>[2x]MSDAAPSLSNLFYDPTYNPGQSTINYTSIYGNGSTITFDELQGLVNSTVTQAIMFGVRCGAAALTLIVMWMTSRSRKTPIFIINQVSLFLIILHSALYFKYLLSNYSSVTYALTGFPQFISRGDVHVYGATNIIQVLLVASIETSLVFQIKVIFTGDNFKRIGLMLTSISFTLGIATVTMYFVSAVKGMIVTYNDVSATQDKYFNASTILLASSINFMSFVLVVKLILAIRSRRFLGLKQFDSFHILLIMSCQSLLVPSIIFILAYSLKPNQGTDVLTTVATLLAVLSLPLSSMWATAANNASKTNTITSDFTTSTDRFYPGTLSSFQTDSINNDAKSSLRSRLYDLYPRRKETTSDKHSERTFVSETADDIEKNQFYQLPTPTSSKNTRIGPFADASYKEGEVEPVDMYTPDTAADEEARKFWTEDNNNL;>[2x]WHWLQLKPGQPMY

The fungal class D1 G-protein-coupled receptor (GPCR) Ste2 has a different arrangement of transmembrane helices compared with mammalian GPCRs and a distinct mode of coupling to the heterotrimeric G protein Gpa1–Ste2–Ste181. Ste2 is a homodimer that can couple to two G proteins simultaneously and its dimer interface is formed by the N terminus, extracellular loop 1 (ECL1) and transmembrane helices H1 and H7. Here we determined structures of Saccharomyces cerevisiae Ste2 in the absence of G protein in two different conformations bound to the native agonist α-factor, bound to an antagonist and without ligand. Activation of Ste2 requires both the removal of a blockage from the G protein coupling site (H7) and formation of the binding site primarily through the inward movement of H6.

The active-state structures of Ste2–Ag were determined bound to the native agonist, pheromone α-factor (WHWLQLKPGQPMY). However, during processing of the Ste2–Ag dataset, two different conformations of Ste2 were found, and therefore two separate structures were determined. By contrast, in the Ste2IL–Ag state (similar to the inactive Ste2–Ant state; the superscript denotes ‘inactive-like’ (IL)), densities for both the N-terminal and C terminal sections are visible in all maps along the principal components, supporting a stronger engagement of Trp1 to cause the shift of the extracellular region of H6 and the rotamer change of Tyr2666x58; by contrast, density in the middle of the peptide was weaker, presumably owing to its flexibility. Ste2–Ant and Ste2–Ag–G represent two extremes in the transition from an inactive state to an active state, and both Ste2IL–Ag and Ste2AL–Ag are consistent with being intermediate states. The cryo-EM density for Ste2IL–Ag and Ste2AL–Ag shows lower resolution in H5–H7 than observed in Ste2–Ant and Ste2–Ag–G, resulting in only a proportion of the side chains being modelled, which highlights their dynamic role in the conformational change. On the extracellular face of the receptor, Ste2IL–Ag has a conformation part way between that of Ste2–Ant and Ste2–Ag–G. This conformation exhibits the agonist-induced displacement of H6 by 5.3 Å (measured at the Cα of Ser2676x59), although this is 0.4 Å short of its position in Ste2–Ag–G, and the reorientation of ECL3. However, there is no significant displacement of the extracellular end of H7 as observed in Ste2–Ag–G and neither are major changes on the intracellular face that are necessary for G protein coupling. These additional structural changes occur in the transition from Ste2IL–Ag to Ste2AL–Ag. Agonist binding to the ligand-free inactive state of Ste2 causes reorientation of the extracellular end of H5 to facilitate ligand binding, an outward movement of the extracellular end of H6 and a shift of ECL3 (Ste2IL–Ag state), resulting in a contraction of the orthosteric binding site by an average of 27%.(4S)-1-methylimidazolidin-4-amine 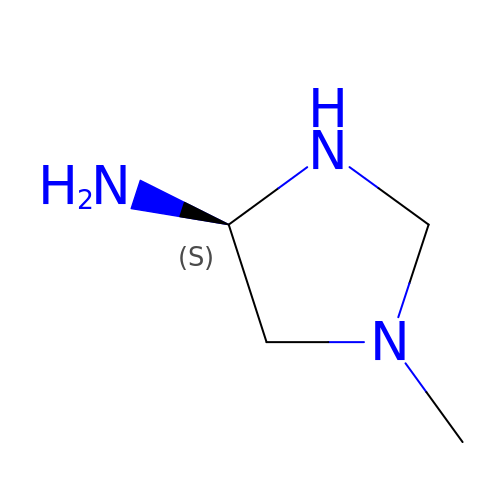| C4 H11 N3 | VFALPSXHULBHMC-BYPYZUCNSA-N Our biochemical and structural analysis of the E. coli MqsA antitoxin and the MqsR:MqsA-N complex provide a detailed 3-dimensional structural view of the free antitoxin and the TA complex. These structures combined with our biochemical data unequivocally demonstrate that MqsR, a protein previously shown to be critical for biofilm formation and the most highly upregulated gene in persister cells in E. coli, and MqsA form a novel bacterial TA system. Our data show that, as expected for a TA system, the expression of the MqsR toxin leads to growth arrest, while co-expression with its antitoxin, MqsA, rescues the growth arrest phenotype. In addition, MqsR associates with MqsA to form a tight, non-toxic complex and both MqsA alone and the MqsR:MqsA2:MqsR complex bind and regulate the mqsR promoter. MqsA itself is a two-domain protein with a novel fold that, unlike every other antitoxin, is well-ordered throughout its entire sequence and whose structure does not change upon toxin binding.

The structure of the MqsR:MqsA-N complex was solved to a resolution of 2.0 Å using the multiple wavelength anomalous dispersion method. The space group of the crystal is P41212, with two crystallographically independent complexes in the asymmetric unit. Moreover, following co-expression, the MqsR:MqsA-N complex is readily purified and forms a heterodimer (one copy of MqsR and one copy of MqsA-N), as determined using size exclusion chromatography, and confirmed using dynamic light scattering. MqsR is a small, globular protein, consisting of a central six-stranded β-sheet (β1-β3-β4-β5-β6-β2) and three α-helices, with α-helix 2 adjacent to and α-helices 1 and 3 abutting the backside of the β-sheet (magenta). The structure of MqsR reveals that it is a member of the RelE/YoeB family of bacterial RNase toxins. MqsA recognition of MqsR occurs at two distinct interfaces. The primary interface is centered on MqsA β-strand 3 (Ser43-Met45), which interacts with MqsR β-strand 2 (Val22-Thr25) to form a single continuous β-sheet (β1R-β3R-β4R-β5R-β6R-β2R-β3A-β2A-β1A) throughout the complex. Finally, MqsA-N does not block the MqsR active site. Instead, nearly all of the residues predicted to be important for MqsR activity are accessible in the MqsR:MqsA-N complex. The only exception is Gln68, which is part of the secondary interface. This suggests neutralization is achieved either through cellular localization (i.e., towards DNA via MqsA-C) or through steric occlusion by blocking the interaction of MqsR with other biomolecules, such as the ribosome.

>MKCPVCHQGEMVSGIKDIPYTFRGRKTVLKGIHGLYCVHCEESIMNKEESDAFMAQVKAFRASVNAETVAPEFIVK[2x];>[2x]GSHMEKRTPHTRLSQVKKLVNAGQVRTTRSALLNADELGLDFDGMCNVIIGLSESDFYKSMTTYSDHTIWQDVYRPRLVTGQVYLKITVIHDVLIVSFKEK4-hydroxyquinoline-3-carboxylic acid | C10 H7 N 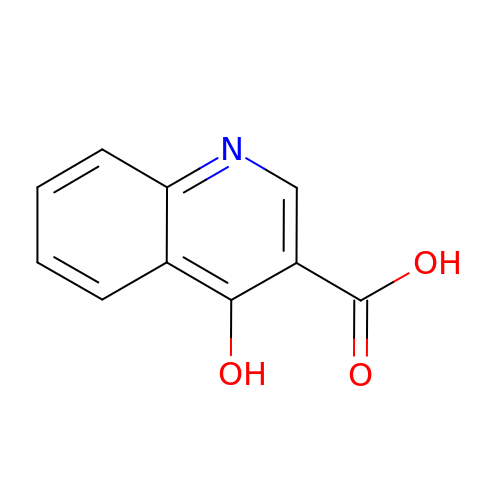O3 | ILNJBIQQAIIMEY-UHFFFAOYSA-N[(2-AMINO-ALPHA-METHOXYIMINO-4-THIAZOLYLACETYL)AMINO]METHYLBORONIC ACID | C7 H11 B N4 O4 S | 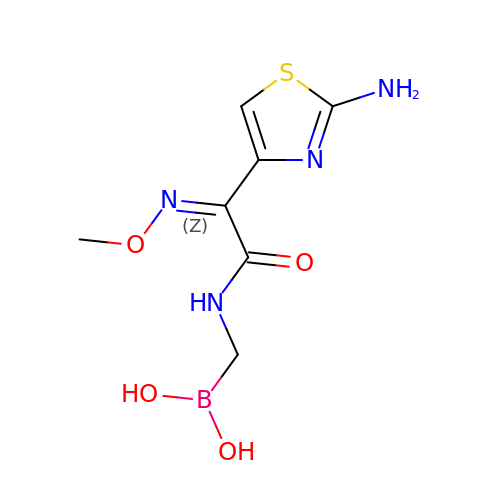FMYGJTQJYFMFCR-XGICHPGQSA-N Human endonuclease VIII-like 1 (hNEIL1) is a bifunctional DNA glycosylase of the Fpg/Nei family, which catalyzes the removal of damaged bases and subsequent incision of the newly generated abasic sites. Unlike traditional enzymes which are commonly referred to as highly specific biocatalysts, one special feature for hNEIL1 is its unique capability to recognize a wide range of substrates, including formamidopyrimidines, hydantoin lesions, oxidized, and dihydro-modified pyrimidine bases, derived from all four canonical bases. Here, by integrating structural, computational, and biochemical investigations, we show that hNEIL1 uses a triage mechanism to achieve broad specificity and reduce futile repair of normal bases. This mechanism involves two mutually competing interaction states: an activated state that commits catalysis and BER, and a quarantine state that temporarily separates and prevents the flipped base from catalysis via auto-inhibition.

While we also crystallized the complex structures for more lesions in this study, we were unable to obtain intact substrates in the active site of hNEIL1, presumably due to the residual glycosylase activity. Hence, we introduced an extra E3Q mutation to the truncated hNEIL1(C∆95 P2G) (see the “Methods” section) and succeeded in the determination of complex structures containing 5-hydroxyuracil (5-OHU), spiroiminodihydantoin 1 (Sp1), (S)-guanidinohydentoin (Gh), dihydrothymine (DHT) and dihydrouracil (DHU), respectively. Despite the very different chemical structures of these substrates, they are recognized similarly by hNEIL1. The damaged bases are fully extruded from the DNA helix and inserted into a relatively loose binding pocket, which allows the accommodation of substrates with varying sizes and shapes. One edge of the flipped base points towards the protein and forms close contact with the side chain of K242. Noteworthy, across all these structures, we observed an unusually short distance (~3.0 Å) between an outwards heterocyclic nitrogen atom of the nucleobases and the terminal nitrogen atom of residue 242. Based on the similar overall conformation and detailed atomic interactions, we conclude that such a tautomerization-dependent mechanism may be a general strategy for hNEIL1 to recognize not only Tg but also 5-OHU, Sp1, Gh, DHT, and DHU. Oxidized substrates of hNEIL1 are often bulky and contain non-planar structures; this disrupted aromaticity is expected to diminish the π–π stacking with Tyr244 and hence destabilize the quarantine state. Moreover, it is expected that the bases with less solvent interactions (e.g. DHU) would favor the formation of a stable quarantine state compared with the hydrophilic bases (Sp1, 5-OHU, Gh, and Tg).

>MGQGPELHLASQFVNEACRALVFGGCVEKSSVSRNPEVPFESSAYRISASARGKELRLILSPLPGAQPQQEPLALVFRFGMSGSFQLVPREELPRHAHLRFYTAPPGPRLALCFVDIRRFGRWDLGGKWQPGRGPCVLQEYQQFRENVLRNLADKAFDRPICEALLDQRFFNGIGNYLRAEILYRLKIPPFEKARSVLEALQQHRPSPELTLSQKIRTKLQNPDLLELCHSVPKEVVQLGGKGYGSESGEEDFAAFRAWLRCYGMPGMSSLQDRHGRTIWFQGDPGPLAPKGRKS[2x]(2S)-N-(2H-1,3-benzodioxol-5-yl)-4-[(isoquinolin-5-yl)sulfonyl]-2-methylpiperazine-1-carboxamide 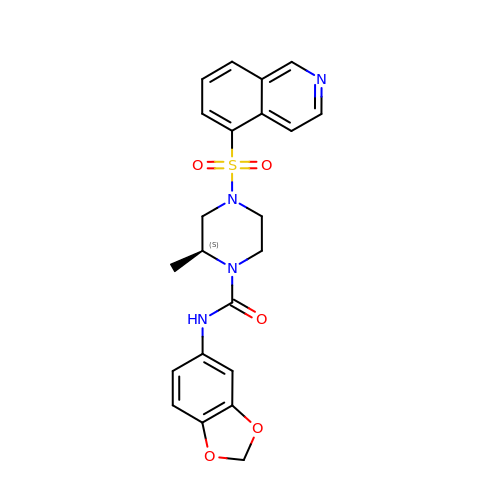| C22 H22 N4 O5 S | JSXIXDYOQGCEHK-HNNXBMFYSA-N> ALRGTVTDFSGFDGRADAEVLRKAMKGLGTDEDSILNLLTARSNAQRQQIAEEFKTLFGRDLVNDMKSELTGKFEKLIVALMKPSRL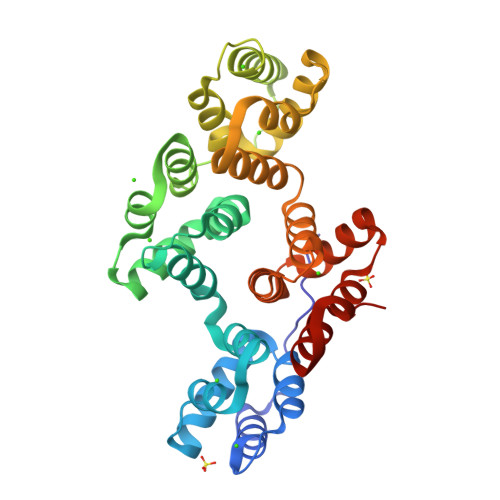YDAYELKHALKGAGTDEKVLTEIIASRTPEELRAIKQAYEEEYGSNLEDDVVGDTSGYYQRMLVVLLQANRDPDTAIDDAQVELDAQALFQAGELKWGTDEEKFITILGTRSVSHLRRVFDKYMTISGFQIEETIDRETSGNLENLLLAVVKSIRSIPAYLAETLYYAMKGAGTDDHTLIRVIVSRSEIDLFNIRKEFRKNFATSLYSMIKGDTSGDYKKALLLLCGGE2-BIPHENYL-4-YL-6-FLUORO-3-METHYL-QUINOLINE-4-CARBOXYLIC 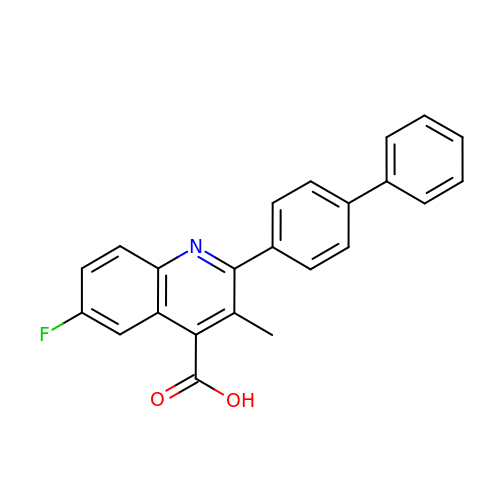ACID | C23 H16 F N O2 | WYKKHJQZENLZID-UHFFFAOYSA-N> MSTFEDADTEETVTCLQMTIYHPGQQSGIFKSIRFCSKEKFPSIEVVKFGRNSNMCQYTFQDKQVSRIQFVLQPFKQFNSSVLSFEIKNMSKKTSLMVDNQELGYLNKMDLPYKCMLRFGEYQFLLQKEDGESVESFETQFIMSSRPLLQENNWPTQNPIPEDGMYSSYFTHRSSPSEMDENELLEHHHHH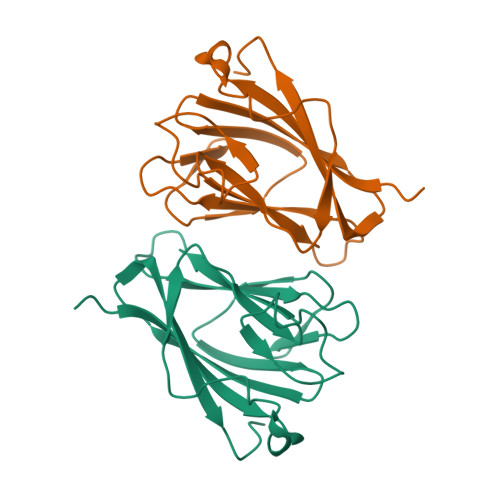H>SGSHMTMGTVNHQPLLTQADLLKRGLADLQEHDAELARILDAEVARQQRTLSLVASCCAVKPRTLAASSSALVNVTAEGVPGRRYHAGCENVDLVESLAIQRARELFGAQYAGVQSHSASSANYQVLAALLEPGDTLLGMALDNGGHLTHGSPVTFSGTYYKAIGYGTTKEGLIDYDEVRRLALEHRPRLIICGATAYSRVVDFERFRQIADEAGAILMADISHIAGLVATGRHPSPIDAAHVTTTCTHKQLVGPRGGLILSGRDANEKVPGRDATFSRVLELAVFPRMQGAPAVNMMAAKAAALGYAMTPEFDAEMQRIRD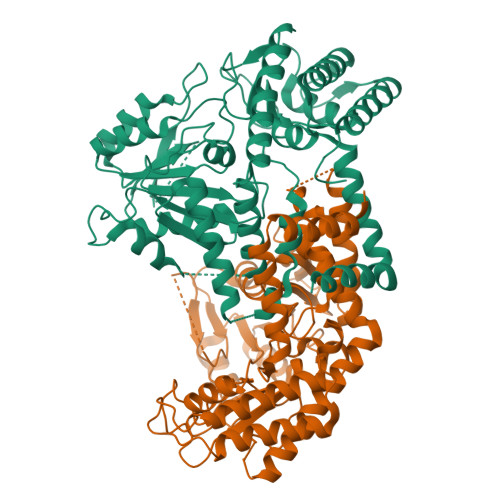AADVMASEFQARDYEVVGGRSENHTILIRLRAAMTGAIAETALEHCGIVVNKNRVPGETRSSFVTSGLRIGTGALAQRHVDAQGCRQIVDLLCRILDEVTPLGESEFTLDPALRKQFCAEAEALCVKYPIADYLAILE[2x]GpsB has emerged as a major regulator of PG biosynthesis in low G+C Gram-positive bacteria, and its homologues (DivIVA/Wag31/antigen 84) in Actinobacteria play essential roles in hyphal growth and branching. To gain molecular understanding of GpsB function, we report three crystal structures of PBP cytoplasmic mini-domains in complex with GpsB, the first structures of a PG synthase in complex with a cytoplasmic cell cycle regulator. The PG synthase arginine finger pokes into a negatively charged cavity situated between α-helices 1 and 2 of GpsB and is fixed in the same orientation in all structures, just as the phosphoryl group defines the binding orientation of peptides to 14-3-345. Therefore, the role of GpsB in the bacterial cell cycle is that of an adaptor, docking PG synthases to other cell wall enzymes, scaffolds and shape determinants into protein complexes for division (the divisome) and peripheral growth (the elongasome).

Since GpsB in both species interact with class A PG synthases, we next determined whether the rules established above for the BsGpsB:BsPBP1 interaction could be applied directly to LmGpsB:LmPBPA1. Therefore, the K32E variant of the N-terminal domain of BsGpsB is as close a surrogate for the equivalent LmGpsB domain that could be obtained. LmPBPA1Arg8 and BsPBP1Arg8 are equivalent in their interactions with GpsB. Of the other GpsB-binding determinants of BsPBP1, LmPBPA1 lacks an analogous BsPBP1Arg11. The sequential equivalent is LmPBPA1Tyr11, but this residue is completely disordered and its mutation to alanine reduced the affinity for BsGpsB1-68Lys32Glu only by 2-fold. LmPBPA11-20Arg8Ala and LmPBPA11-20Arg12Ala mutations reduced the affinity for BsGpsB1-68Lys32Glu by >15- and ~4-fold, respectively, and had significant negative impact on the LmGpsB:LmPBPA1 interaction by BACTH. Reintroducing positive charge into LmPBPA11-20Arg8Ala did not restore wild-type binding affinity in FP as LmPBPA11-20Arg8Ala,Ser16Arg still bound to BsGpsB1-68Lys32Glu with an affinity at least 10-fold weaker than wild-type. It would thus seem that LmPBPA1 represents the only GpsB binding partner that employs the TRxxYR motif in L. monocytogenes.

>GHMKVKLSAKEILEKEFKTGVRGYKQEDVDEFLDMIIKDYETFHQEIEELQQENLQLKKQLEE[2x];> MADKPQTRSQYRNKQ>MHHHHHHMAKYEATKGDYAGGVLAILTQY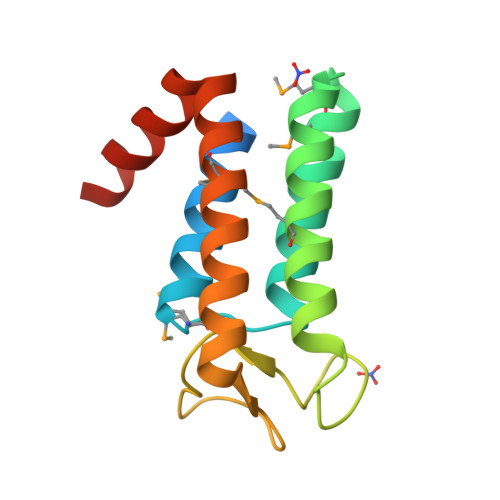FNNMVGYPEVSLKLAGEEANMSREGMINQKEIVHQMVETIRRASEPIRQGRGFHDAYVYFASVPENAPPNSIALPPQAQSEVQAKLTELMQKLANRNPQGVAEEEQELATQGI[5x]> MPAHYISDIAQQREGHEAAADFLDIFSHRLITQYYRIWRKYSYPATFEAGGQDKTSQYLLGLARLGIPGCAQNIATPVSRFLALLPLMLLPGRTAEGLTSLVTLLAPGTQARVWHHDRRRIPLKTPLTMRVHHPVSLKSRPVMGDHATDVNGQVLLQLSTQTGSEVQGWLPGGHLYSDLLALLHVYLGSRLDVRLQLCVERSLLPDARLSCRPAAGSPQLGRTAVMRTQAKITTSAARVMTISLGRYQRVQEHYQRKETQENGDYRW;>[6x]MKIYRPLWEDGAFLMPQQFQQQAAWDVHLADSVARMGLAHPWGVVAAEFDDSLLPLSRLNATRLIVRFPDGTLIDTERADNLPPVCDL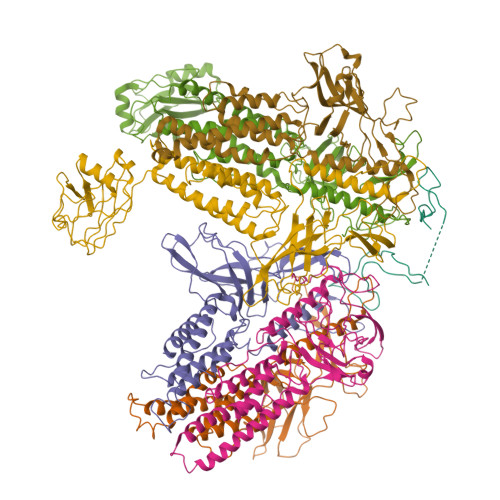STVSDRSLVDIVLALPLLNANGGNLDNGSESERPRRWKSERVNVQELAGHEQSEVAVLRHNLTLRMAHQENAAWLTCPVTRLVRDAQGQWCRDPRFIPPLLTLSASPSLMTELLELLHHLQARRQRLMSMRRENNARLADFAVADVSLFWLLNALNSAEPVLKELLDMPYRHPELLYRELARLAGSLLTFSLEHNVDAVPAYHHETPENVFPPLLSLLNRLLEASLPSRVVFIELKQKGVMWEGALHDARLREGADFWLSVRSSMPGHELQTKFPQLCKAGSPDDVSEVVNVALSGVIIRPVTHVPAAIPLRLENQYFALDLSTDAARAMLDAGRCTFYTPASLGDVKLELFAVLRT The LpxH enzyme cleaves the pyrophosphate bond of UDP-2, 3-bis(3-hydroxytetradecanoyl)-glucosamine (UDP-DAGn) to yield lipid X (PubChem CID 123907) and UMP in the fourth step of lipid A biosynthesis. Roughly 70% of Gram-negative bacteria, including the WHO critical priority Gram-negative pathogens for R&D of new antibiotics, utilize this enzyme. The importance of LPS, and lipid A in particular, for the viability and virulence of Gram-negative bacteria makes the inhibition of lipid A biosynthesis a promising target for the development of antibiotics. To enable a structure-based drug design approach for the optimization of JEDI-1444, we produced LpxH proteins from E. coli (EcLpxH) and K. pneumoniae (KpLpxH) and solved the X-ray crystal structures of various enzyme-product and inhibitor complexes during the optimization of the chemical series.

As for HiLpxH, the EcLpxH and KpLpxH proteins copurified with a bound molecule of lipid X in the substrate binding site but we were able to develop protocols to displace the product and form enzyme–inhibitor complexes. The 1.35-Å resolution EcLpxH complex, in particular, provides a detailed view of this portion of the substrate-binding site. In contrast to the highly mutated EcLpxH structure previously published, the lid of our structure is generally well-ordered. One of the lipid X aliphatic tails extends toward the protein surface and is partially solvent-exposed, while the other is completely buried in the enzyme interior. The nonpolar side chains that interact with this buried aliphatic chain are conserved in EcLpxH and KpLpxH, producing a roughly 120° bend in the aliphatic chain. Indeed, the binding of the lipid X product to EcLpxH and PaLpxH structures shows differences at the ring 1-binding site that would be expected to affect inhibitor binding.

> MATLFIADLHLCVEEPAITAGFLRFLAEEARKADALYILGDLFEAWIGDDDPNPLHRQMAAAIKAVSDSGVPCYFIHGNRDFLLGKRFARESGMTLLPEEKVLELYGRRVLIMHGDTLCTDDAGYQAFRAKVHKPWLQMLFLALPLFVRKRIAARMRANSKEANSSKSLAIMDVNQNAVVSAMEKHQVQWLIHGHTHRPAVHELIANQQPAFRVVLGAWHTEGSMVKVTADDVELIHFPFHHHHHH>[2x]MASWSHPQFEKGAETAVMNILFIMFDQLRWDYLSCYGHKTLNTPHIDRLAAKGVRFDRAYIQSPICGSSRMSTYTGRYVHSHGASWNGIPLKVGEMTMGDHLRAAGMGCWLVGKTHMRADEEGMARLGLEPDSLIGARVAECGFDVFERDDGMLPEGPDGYYDPDGAKEYNKFLRAKGYESDNPWHDFANSGLDDEGNVQSGWFLKNATRPANIAEEDSETPYLTSRAMEFIEQQTGPWCCHLSYIKPHWPYIVPEPYASMFGPEHVQDVVRSDSERQNAHPLFKAFMDTKVGEAFSRQEVRDAVIPAYMGLIKQADDQMGRLFKWLEDTGRMQDTMIVLTSDHGDF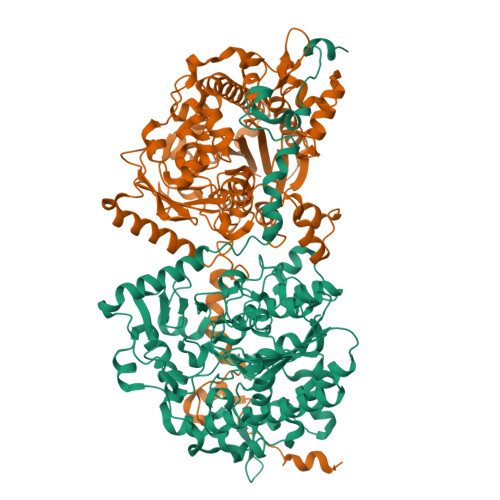LGDHWMGEKTFFHDASTRVPLIIYDPRPEADATRGSVCDALVESIDLAPTFVEAAGGKPAMHILEGESLIPILHGARDHTLRDHVICEYDFSASPIAHLNDISVRQAVMFMVADKNWKLIHFEADPRPMLFDLKNDPQELVDLGGDPAHADVIAGMYDKLFRWTRRQSQRTTRSEEQLIAMRTKSRKRGIVLGIYDENETPLELTVKYRDRKARPYKDYLKG> RALAAPLVHHHHHHALDENLYFQGALADVSRPPHARKTGGSSPETKYDQPPKCDISGKEAISALSRAKSKHCRQEIGETYCRHKLGLLMPEKVTRFCPLEGKANKNVQWDEDSVEYMPANPVRIAFVLVVHGRASRQLQRMFKAIYHKDHFYYIHVDKRSNYLHRQVLQVSRQYSNVRVTPWRMATIWGGASLLSTYLQSMRDLLEMTDWPWDFFINLSAADYPIRTNDQLVAFLSRYRDMNFLKSHGRDNARFIRKQGLDRLFLECDAHMWRLGDRRIPEGIAVDGGSDWFLLNRRFVEYVTFSTDDLVTKMKQFYSYTLLPAESFFHTVLENSPHCDTMVDNNLRITNWNRKLGCKCQYKHIVDWCGCSPNDFKPQDFHRFQQTARPTFFARKFEAVVNQEIIGQLDYYLYGNYPAGTPGLRSYWENVYDEPDGIHSLSDVTLTLYHSFARLGLRRAETSLHTDGENSCRYYPMGHPASVHLYFLADRFQGFLIKHHATNLAVSKLETLETWVMPKKVFKIASPPSDFGRLQFSEVGTDWDAKERLFRNFGGLLGPMDEPVGMQKWGKGPNVTVTVIWVDPVNVIAATYDILIESTAEFTHYKPPLNLPLRPGVWTVKILHHWVPVAETKFLVAPLTFSNRQPIKPEEALKLHNGPLRNAYMEQSFQSLNPVLSLPINPAQVEQARRNAASTGTALEGWLDSLVGGMWTAMDICATGPTACPVMQTCSQTAWSSFSPDPKSELGAVKPDGRLR;> QEEEGSGGGQGG

The first enzyme in the pathway, peptide O-xylosyltransferase (XT, EC 2.4.2.26), catalyzes the transfer of xylose from uridine diphosphate (UDP)-α-D-xylose onto serine and thus determines the site(s) of GAG attachment on the core protein. XT1 and XT2 are type II transmembrane proteins consisting of a short amino-terminal region facing the cytosol, a single transmembrane helix, a stem region required for Golgi localization (Schön et al., 2006), a catalytic GT-A domain (Lairson et al., 2008, Müller et al., 2006), and a unique C-terminal domain of unknown function, termed “Xylo_C” in the Pfam database (Finn et al., 2008). XT1 has a two-lobed structure, with one lobe comprising the catalytic GT-A domain and the other comprising the Xylo_C domain. To better understand the initial step of GAG biosynthesis, we have determined crystal structures of human XT1 complexed with UDP-xylose and various PG-derived acceptor peptides.

To obtain defined complexes, we used crystal soaking to replace the co-purified ligand with dodecapeptides derived from the PGs bikunin and syndecan 1. Peptides 1 and its variants (2 to 7) are derived from bikunin. Superposition of the binary complex with active peptide 1 and the ternary complex with inactive peptide 2 allowed us to construct a model of the Michaelis complex. In this model, the serine OH group is perfectly positioned for nucleophilic attack on the UDP-xylose C1 carbon atom. When the XT1 complex with peptide 1 is compared with the C2GnT-L complex with the acceptor Gal-β1,3-GalNAc (Pak et al., 2006), the attacking oxygen atoms occupy the same position. Thus, we believe that we have crystallized a catalytically competent conformation of XT1. Indeed, when we soaked XT1 crystals with UDP-xylose and catalytically active peptide 1, the electron density for the xylose group disappeared, presumably due to GT activity within the crystal (not shown). From our structures, we estimate that at least four residues either side of the serine need to be in an extended conformation to fit into the active-site cleft of XT1.> MVMNKQIVLNNYINGSLKQSDLALRTSTICMEIPDGCNGAILVKNLYLSVNPYLILRMGKLDIPQFDSILPGSTIVSYGVSKVLDSTHPSYEKGELIWGSQAGWEEYTLIQNPYNLFKIQDKDVPLS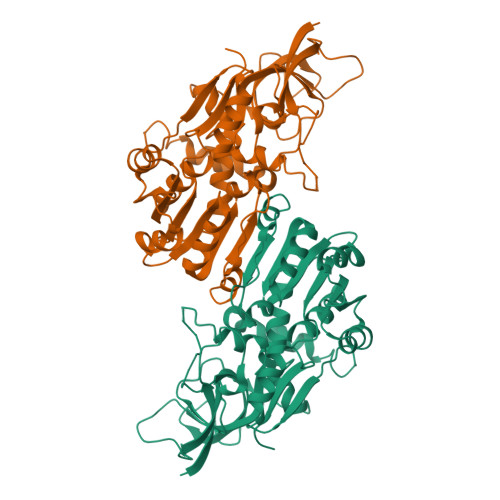YYVGILGMPGMTAYAGFFEICSPKKGETVFVTAAAGSVGQLVGQFAKMFGCYVVGSAGSKEKVDLLKNKFGFDDAFNYKEESDYDTALKRHFPEGIDIYFDNVGGKMLEAVINNMRVHGRIAVCGMVSQYSLKQPEGVHNLLKLIPKQIRMQGFVVVDYYHLYPKFLEMVLPRIKEGKVTYVEDISEGLESAPSALLGVYVGRNVGNQVVAVSRE> MASPALQTCWRNLARLSGAQVRPSHFGAFSLGSRMSPFSSLLGARASPIATGRAGLRFLSSAAPNPGKKPASAAPPAGTNHGRITQVIGAVVDVHFDEQLPPILNSLEVQGHTNRLVLEVAQHLGENTVRTIAMDATEGLVRGQKVVDTGAPIQVPVGVETLGRIMNVIGEPVDECGPVPAKKTYSIHRAAPLFADQSTEPGLLQTGIKVVDLLAPYAKGGKIGLFGGAGVGKTVLI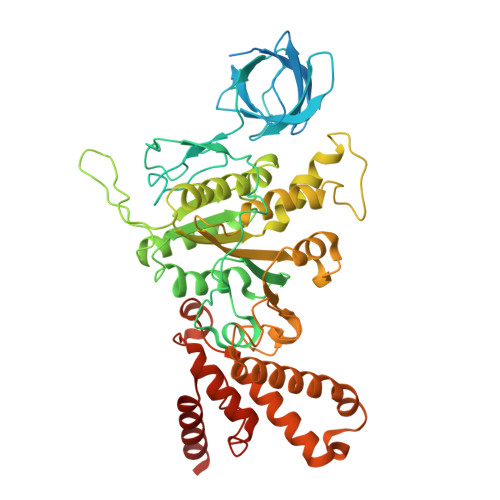MELINNVANKHGGFSVFAGVGERTREGNDLYHEMMTTGVIKRKKLEDGKFDFTGSKAALVYGQMNEPPGARARVALTALSVAEYFRDEQGQDVLLFIDNIYRFTQAGSEVSALLGRIPSAVGYQPTLATDLGQLQERITTTKKGSITSVQAVYVPADDLTDPAPATTFAHLDATTVLSRQIAELGIYPAVDPLDSTSRMLAPEIVGQEHYDTARATQKLLQDYKSLQDIIAILGMDELSEEDKLVVSRARKIQRFLSQPFTVAEVFTGKPGRFVELPETIKSAQTILRGECDDLPEMAFYMCGGLEEVRSKAVKMAQEAASGK> WYTPPSKRTWSKQHNKIFTPRPLSERFSPHKLHPEFEWWRERTVQPSALFMGFPDLLALPLRGGSAYIHEMDAATLAVVLASLAHSPSAYSVSERRPPPSPSPAVSLSSSSFSPTHLPQHLDSLLALLGRQAAATAAHAPDSTLAFLFRGCAEAGVVEKNVVCTLLGRVEQRLPCMQLPECLVLLDALRPGLPEVYRHPRFVARLVAHAGLLLQFRGAESEAEDLCDLAFSLVFAANCRDAALLQTTALLLVHGKRMQSLNETAPLALARAMEAFAACRDAVNAPLLAETAAAAENGDAEGSRNTKAAELFCASPLLRAREPSVHLSPSGWLLLSLLSPVVQALHRAEKGRRKRRGFHQDG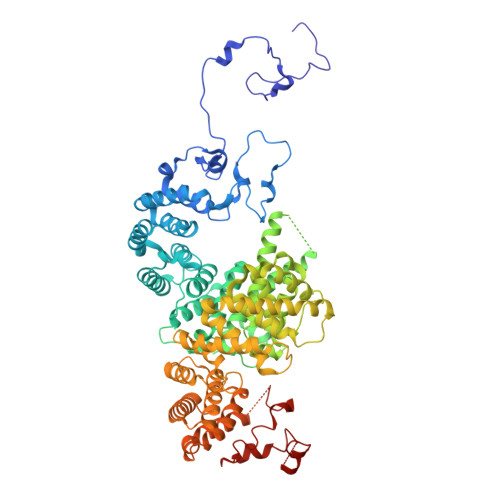EAAGLTAEREVQNRGASRESHALTEAAARAAAAVAEETQTLKNRESSLFRGLLRCLERVDDHRESLSPGSMCKVLFAATVARAAPSRDFFPDVLKRLGDQLGACTPEDLSRALFALVKLSSVSGLDPRCQDLLPPLLGTVLQAVESSLPVADVASLARLHSAAVSALISSSETKKEEMKQLAEETSRLMHARLEEASPAHLTAFVRHWDLVPAPSGAFREALVAQAIRQLYFFDEDHLSRLLEGVTRLAASSKDETLLASVDELFRRAEEEATTEQAFFSPESCLRIFVSLVRYGEVRPEAPRNRERLVVALCNYLTGVDSVAAVSSDGASDPEELWVKEDEDLPLLFFAEDAKGFSLREDSALDRDSANESRLQALSAASYIRLLGALRELGVRGGVLLSRVAQLLHMKRYDLTDAQQEAAAEIC> MFQQLSARLQEAIGRLRGRGRITEEDLKATLREIRRALMDADVNLEVARDFVERVREEALGKQVLESLTPAEVILATVYEALKEALGGEARLPVLKDRNLWFLVGLQGSGKTTTAAKLALYYKGKGRR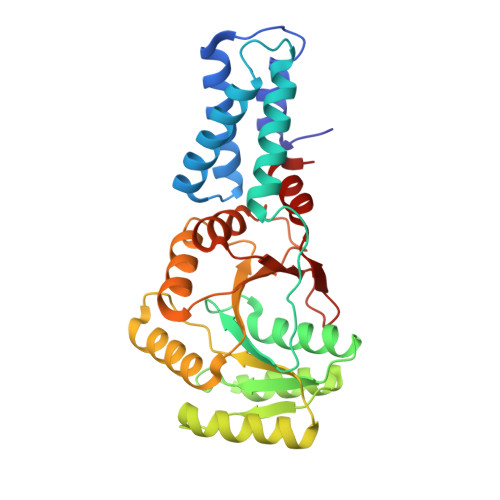PLLVAADTQRPAAREQLRLLGEKVGVPVLEVMDGESPESIRRRVEEKARLEARDLILVDTAGRLQIDEPLMGELARLKEVLGPDEVLLVLDAMTGQEALSVARAFDEKVGVTGLVLTKLDGDARGGAALSARHVTGKPIYFAGVSEKPEGLEPFYPERLAGRILGM> ERLTLPPSEIT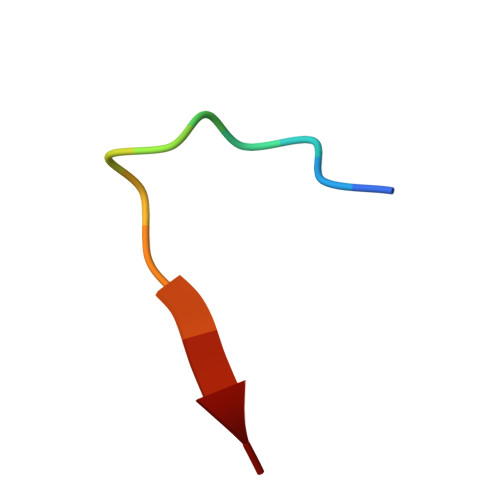LL>MASEIHMTGPMCLIENTNGRLMANPEALKILSAITQPMVVVAIVGLYRTGKSYLMNKLAGKKKGFSLGSTVQSHTKGIWMWCVPHPKKPGHILVLLDTEGLGDVEKGDNQNDSWIFALAVLLSSTFVYNSIGTINQQAMDQLYYVTELTHRIRSKSSPDENENEVEDSADFVSFFPDFVWTLRDFSLDLEADGQPLTPDEYLTYSLKLKKGTSQKDETFNLPRLCIRKFFPKKKCFVFDRPVHRRKLAQLEKLQDEELDPEFVQQVADFCSYIFSNSKTKTLSGGIQVNGPRLESLVLTYVNAISSGDLPCMENAVLALAQIENSAAVQKAIAHYEQQMGQKVQLPTETLQELLDLHRDSEREAIEVFIRSSFKDVDHLFQKELAAQLEKKRDDFCKQNQEASSDRCSALLQVIFSPLEEEVKAGIYSKPGGYRLFVQKLQDLKKKYYEEPRKGIQAEEILQTYLKSKESMTDAILQTDQTLTEKEKEIEVERVKAESAQASAKMLQEMQRKNEQMMEQKERSYQEHLKQLTEKMENDRVQLLKEQERTLALKLQEQEQLLKEGFQKESRIMKNEIQDLQTKMRRRKACTIS[2x]

Guanylate-binding proteins (GBPs) are interferon-inducible guanosine triphosphate hydrolases (GTPases) mediating host defense against intracellular pathogens. Their antimicrobial activity hinges on their ability to self-associate and coat pathogen-associated compartments or cytosolic bacteria. GBP1 is a multidomain protein consisting of an N-terminal large GTPase (LG) domain and a C-terminal α-helical region (C-terminal helical domain, CTHD), divided into a middle domain (MD; α7–α11) and an elongated C-terminal GTPase effector domain (GED; α12–α13). In the absence of guanine nucleotides, the GED folds onto the MD and interacts with the LG domain and MD to maintain GBP1 in the resting state.

Unlike the isolated LG domain that readily dimerizes under several guanine nucleotide conditions, full-length GBP1 forms stable dimers only in the presence of GDP·AlF3. We next determined the 3D structure of Nb74-bound GBP1 dimers in complex with GDP·AlF3, yielding a pseudo-C2 symmetric 3D reconstruction at a nominal resolution of 3.7 Å. GBP1 associates through the LG domains and additional contacts between the MDs, which extend in parallel from the LG dimer in a crossover arrangement mediated by the Gly307–Val316 linker region connecting the LG domain and MD. Nucleotide binding induced partial unraveling of the C-terminal part of helix α6 (Ile304–Ser306) and the N-terminal end of helix α7 (Cys310–Val316) to form the crossover interface, in which the MD swings out to form contacts with the respective pairing monomer. This interface is primarily formed by a hydrophobic patch between the LG domain of one monomer and an aliphatic stretch of residues at the C-terminal end of the linker region and helix α7 (Ala315–Ile322) in the other monomer. While the MDs undergo a large spatial transformation relative to the resting state, the overall conformation of helices α7–α11 remains essentially unchanged with a root-mean-square deviation (r.m.s.d) of 2.03 Å relative to the nucleotide-free state. The parallel arrangement of the MD is stabilized by an electrostatic zipper along α9–α11 of the protruding stalks. The GED (residues 481–592) is likely flexible and not visible in our structure. Our structure was obtained with recombinant protein devoid of the farnesyl modification normally required for association with membranes. In this structure, the MDs point away in parallel from the LG domains, compatible with a model in which nucleotide binding primes both farnesyl anchors for membrane insertion.1-methyl-8-[(oxan-4-yl)methyl]-3-[4-(trifluoromethyl)phenyl]-1,3,8-triazaspiro[4.5]decane-2,4-dione 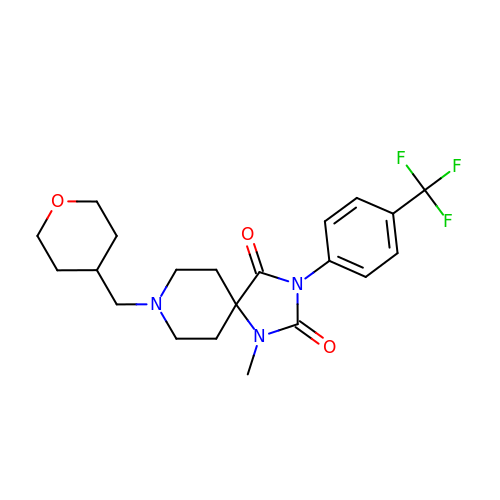| C21 H26 F3 N3 O3 | PGRXOQYVDWCZAG-UHFFFAOYSA-N>EGAALTEKTDIFESGRNGKPNKDGIKSYRIPALLKTDKGTLIAGADERRLHSSDWGDIGMVIRRSEDNGKTWGDRVTITNLRDNPKASDPSIGSPVNIDMVLVQDPETKRIFSIYDMFPEGKGIFGMSSQKEEAYKKIDGKTYQILYREGEKGAYTIRENGTVYTPDGKATDYRVVVDPVKPAYSDKGDLYKGNQLLGNIYFTTNKTSPFRIAKDSYLWMSYSDDDGKTWSAPQDITPMVKADWMKFLGVGPGTGIVLRNGPHKGRILIPVYTTNNVSHLNGSQSSRIIYSDDHGKTWHAGEAVNDNRQVDGQKIHSSTMNNRRAQNTESTVVQLNNGDVKLFMRGLT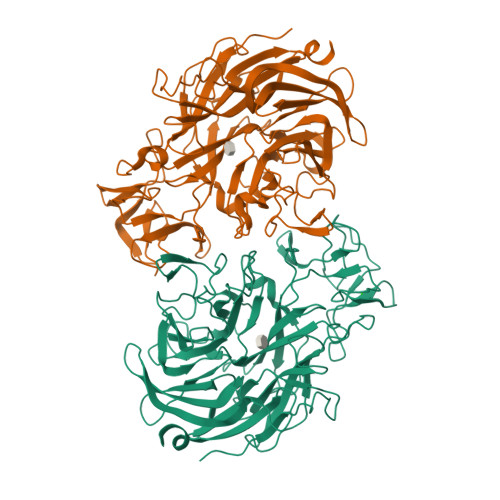GDLQVATSKDGGVTWEKDIKRYPQVKDVYVQMSAIHTMHEGKEYIILSNAGGPKRENGMVHLARVEENGELTWLKHNPIQKGEFAYNSLQELGNGEYGILYEHTEKGQNAYTLSFRKFNWDFLSKDLISPTEAKVKRTREMGKGVIGLEFDSEVLV[2x]>[2x]MNGAIKVGAWGG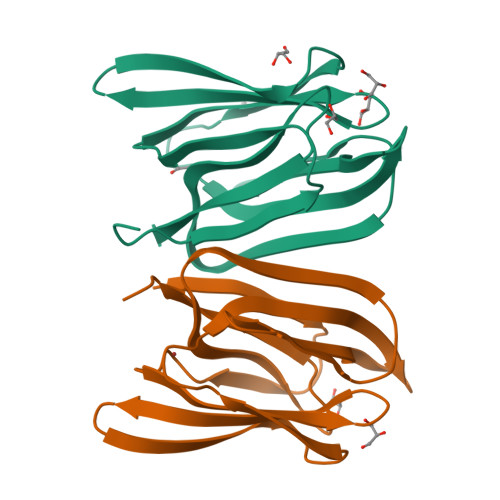NGGSAFDMGPAYRIISVKIFSGDVVDGVDVTFTYYGKTETRHYGGSGGTPHEIVLQEGEYLVGMAGEVANYHGAVVLGKLGFSTNKKAYGPFGNTGGTPFSLPIAAGKISGFFGRGGKFLDAIGVYLEPASGENLYFQ> MGLLSDPVRRRALARLVLRLNAPLCVLSYVAGIAWFLALVFPPLTQRTYMSENAMGSTMVEEQFAGGDRARAFARDFAAHRKKSGALPVAWLERTMRSVGLEVYTQSFSRKLPFPDETHERYMVSGTNVYGILRAPRAASTESLVLTVPCGSDSTNSQAVGLLLALAAHFRGQIYWAKDIVFLVTEHDLLGTEAWLEAYHDVNVTGMQSSPLQGRAGAIQAAVALELSSDVVTSLDVAVEGLNGQLPNLDLLNLFQTFCQKGGLLCTLQGKLQPEDWTSLDGPLQGLQTLLLMVLRQASGRPHGSHGLFLRYRVEALTLRGINSFRQYKYDLVAVGKALEGMFRKLNHLLERLHQSFFLYLLPGLSRFVSIGLYMPAVGFLLLVLGLKALELWMQLHEAGMGLEEPGGAPGPSVPLPPSQGVGLASLVAPLLISQAMGLALYVLPVLGQHVATQHFPVAEAEAVVLTLLAIYAAGLALPHNTHRVVSTQAPDRGWMALKLVALIYLALQLGCIALTNFSLGFLLATTMVPTAALAKPHGPRTLYAALLVLTSPAATLLGSLFLWRELQEAPLSLAEGWQLFLAALAQGVLEHHTYGALLFPLLSLGLYPCWLLFWNVLFWK;> MAVTDSLSRAATVLATVLLLSFGSVAA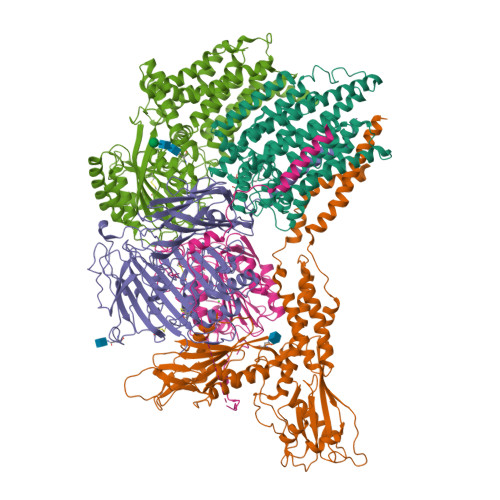SHIEDQAEQFFRSGHTNNWAVLVCTSRFWFNYRHVANTLSVYRSVKRLGIPDSHIVLMLADDMACNPRNPKPATVFSHKNMELNVYGDDVEVDYRSYEVTVENFLRVLTGRIPPSTPRSKRLLSDDRSNILIYMTGHGGNGFLKFQDSEEITNIELADAFEQMWQKRRYNELLFIIDTCQGASMYERFYSPNIMALASSQVGEDSLSHQPDPAIGVHLMDRYTFYVLEFLEEINPASQTNMNDLFQVCPKSLCVSTPGHRTDLFQRDPKNVLITDFFGSVRKVEITTETIKLQQDSEIMESSYKEDQMDEKLMEPLKYAEQLPVAQIIHQKPKLKDWHPPGGFILGLWALIIMVFFKTYGIKHMKFIF;> AATHLEVARGKRAALFFAAVAIVLGLPLWWKTTETYRASLPYSQISGLNALQLRLMVPVTVVFTRESVPLDDQAKLPFTVVHEREIPLKYKMKIKCRFQKAYRRALDHEEEALSSGSVQEAEAMLDEPQEQAEGSLTVYVISEHSSLLPQDMASYIGPKRTAVVRGIMHREAFNIIGRRIVQVAQAMSLTEDVLAAALADHLPEDKWSAEKRRPLKSSLGYEITFSLLNPDPKSHDVYWDIEGAVRRYVQPFLNALGAAGNFSVDSQILYYAMLGVNPRFDSASSSYYLDMHSLPHVINPVESRLGSSAASLYPVLNFLLYVPELAHSPLYIQDKDGAPVATNAFHSPRWGGIMVYNVDSKTYNASVLPVRVEVDMVRVMEVFLAQLRLLFGIAQPQLPPKCLLSGPTSEGLMTWELDRLLWARSVENLATATTTLTSLAQLLGKISNIVIKDDVASEVYKAVAAVQKSAEELASAHLASAFVASQEAVTSSELAFFDASLLHLLYFPDDQKFAIYIPLFLPMAVPILLSLVK;> ARDSLREELVITPLPSGDVAATFQFRTRWDSELQREGVSHYRLFPKALGQLISKYSLRELHLSFTQGFWRTRYWGPPFLQAPSGAELWVWFQDTVTDVDKSWKELSNVLSGIFCASLNFIDSTNTVTPTASFKPLGLANDTDHYFLRYAVLPREVVCTENLTPWKKLLPCSSKAGLSVLLKADRLFHTSYHSQAVHIRPVCRNARCTSISWELRQTLSVVFDAFITGQGKKDWSLFRMFSRTLTEPCPLASESRVYVDITTYNQDNETLEVHPPPTTTYQDVILGTRKTYAIYDLLDTAMINNSRNLNIQLKWKRPPENEAPPVPFLHAQRYVSGYGLQKGELSTLLYNTHPYRAFPVLLLDTVPWYLRLYVHTLTITSKGKENKPSYIHYQPAQDRLQPHLLEMLIQLPANSVTKVSIQFERALLKWTEYTPDPNHGFYVSPSVLSALVPSMVAAKPVDWEESPLFNSLFPVSDGSNYFVRLYTEPLLVNLPTPDFSMPYNVICLTCTVVAVCYGSFYNLLTRTFH;> MAAPLVLVLVVAVTVRAALFRSSLAEFISERVEVVSPLSSWKRVVEGLSLLDLGVSPYSGAVFHETPLIIYLFHFLIDYAELVFMITDALTAIALYFAIQDFNKVVFKKQKLLLELDQYAPDVAELIRTPMEMRYIPLKVALFYLLNPYTILSCVAKSTCAINNTLIAFFILTTIKGSAFLSAIFLALATYQSLYPLTLFVPGLLYLLQRQYIPVKMKSKAFWIFSWEYAMMYVGSLVVIICLSFFLLSSWDFIPAVYGFILSVPDLTPNIGLFWYFFAEMFEHFSLFFVCVFQINVFFYTIPLAIKLKEHPIFFMFIQIAVIAIFKSYPTVGDVALYMAFFPVWNHLYRFLRNIFVLTCIIIVCSLLFPVLWHLWIYAGSANSNFFYAITLTFNVGQILLISDYFYAFLRREYYLTHGL> PVVKTAQNLAEVNGPETLIGPGAKEGTVPTDLDQETGLARLELLGKLEGIDV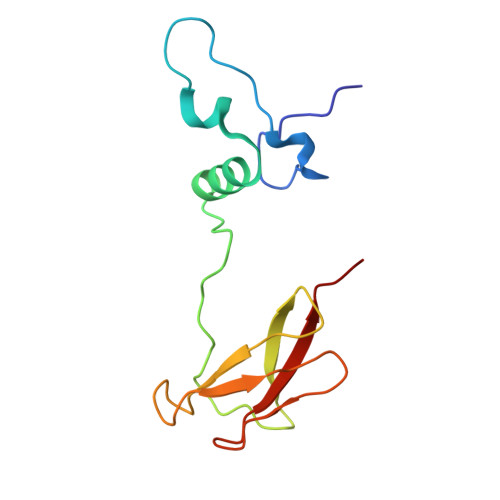FDTKPLDSSRKGTMKDPIIIESYDDYRYVGCTGSPAGSHTIMWLKPTVNEVARCWECGSVYKLNPVGVP>GSHMTEGTIKTSKYEIIAIFREELRKRTEIEIFFNNTSIITQLTRVDFAEFHIQTHRKIPSGHKIRFLLHSDSGKIEFNAALTKHDNSGVDKGIRYAFSLPECLQVVQRRRDPRFRLRHEHDFYCRGRHKNGENYLFDIKDISDGGCALMTKTPNLKFLSHNALLKNAVLMLAEYGEITIDLVVKNVIVITLDNANEESESYYQISCQF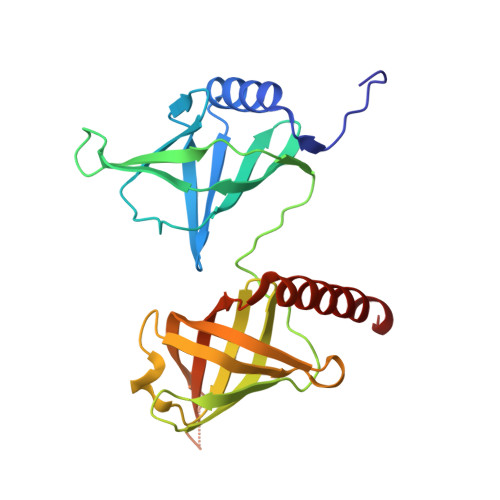KFRHLDDQRRIEKILLDLILEAKRKK[4x]>AAAAAAMTMMDMNFKYCHKIMKKHSKSFSYAFDLLPEDQRKAVWAIYAVCRKIDDSIDVYGDIQFLNQIKEDIQSIEKYPYEYHHFQSDRRIMMALQHVAQHKNIAFQSFYNLIDTVYKDQHFTMFETDAELFGYCYGVAGTVGEVLTPILSDHETHQ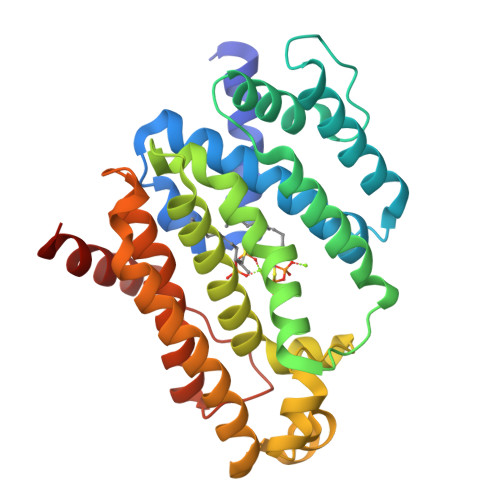TYDVARRLGESLQLINILRDVGEDFENERIYFSKQRLKQYEVDIAEVYQNGVNNHYIDLWEYYAAIAEKDFRDVMDQIKVFSIEAQPIIELAARIYIEILDEVRQANYTLHERVFVEKRKKAKLFHEINSKYHRI[2x]>[2x]MTSALIERIDAIIVDLPTIRPHKLAMHTMQQQTLVVLRVRCSDGVEGIGEATTIGGLAYGYESPEGIKANIDAHLAPALIGLAADNINAAMLKLDKLAKGNTFAKSGIESALLDAQGKRLGLPVSELLGGRVRDSLEVAWTLASGDTARDIAEARHMLEIRRHRVFKLK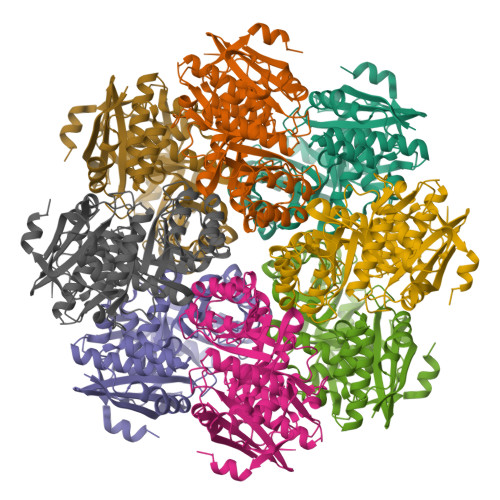IGANPVEQDLKHVVTIKRELGDSASVRVDVNQYWDESQAIRACQVLGDNGIDLIEQPISRINRGGQVRLNQRTPAPIMADESIESVEDAFSLAADGAASIFALKIAKNGGPRAVLRTAQIAEAAGIGLYGGTMLEGSIGTLASAHAFLTLRQLTWGTELFGPLLLTEEIVNEPPQYRDFQLHIPRTPGLGLTLDEQRLARFARR> MHPGFFTSIGQMTDLIHTEKDLVTSLKDYIKAEEDKLEQIKKWAEKLDRLTSTATKDPEGFVGHPVNAFKLMKRLNTEWS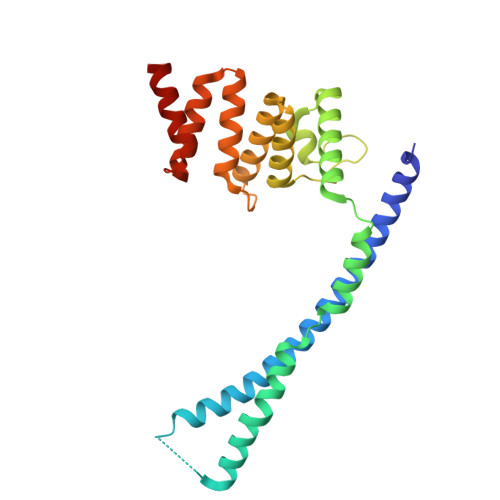ELENLVLKDMSDGFISNLTIQRQYFPNDEDQVGAAKALLRLQDTYNLDTDTISKGNLPGVKHKSFLTAEDCFELGKVAYTEADYYHTELWMEQALRQLDEGEISTIDKVSVLDYLSYAVYQQGDLDKALLLTKKLLELDPEHQRANGNLKYFEYIMAKE>SNAMIPAKLKQGDEIRIIAPSRSIGIMADNQVEIAVNRLTDMGFKVTFGEHVAEMDCMMSSSIRSRVADIHEAFNDSSVKAILTVIGGFNSNQLLPYLDYDLISENPKILCGFADITALATAIYTQTELITYSGAHFSSFSMEKGLDYVMESFSDCLLQKEPFALKESATWSDDEWYLDQENRNFIPNEGLVVMQPGVAE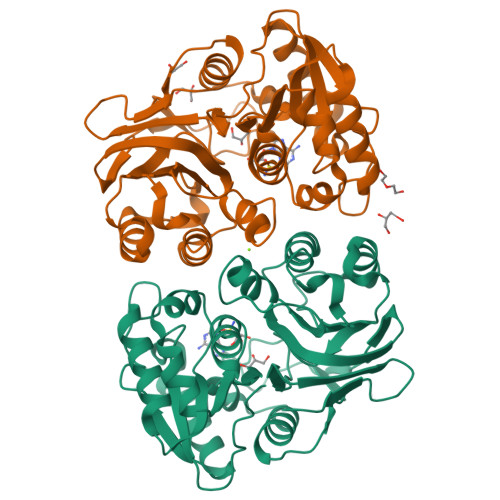GIIIGGNLCTLNLLQGTEYMPNLAGTILFIEDDFMTIPETFDRDLESLLSQPGADEIEGMVIGRFQQKTAMTAEKLAYIIETKTALQKIPVISGADFGHTQPIATFPIGGTARIDTNQTDKIQIIRH[2x]>[2x]EPCVEVVPNITYQCMELNFYKIPDNLPFSTKNLDLSFNPLRHLGSYSFFSFPELQVLDLSRCEIQTIEDGAYQSLSHLSTLILTGNPIQSLALGAFSGLSSLQKLVAVETNLASLENFPIGHLKTLKELNVAHNLIQSFKLPEYFSNLTNLEHLDLSSNKIQSIYCTDLRVLHQMPLLNLSLDLSLNPMNFIQPGAFKEIRLHKLTL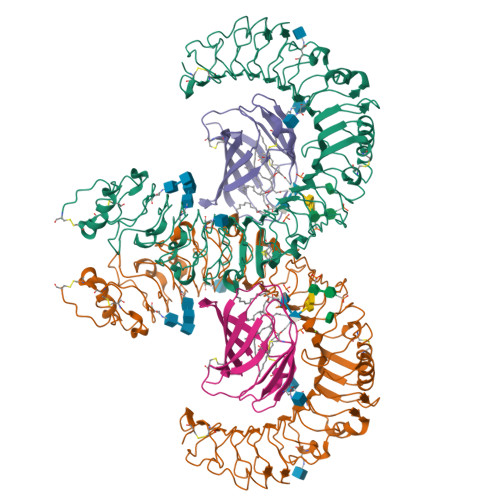RNNFDSLNVMKTCIQGLAGLEVHRLVLGEFRNEGNLEKFDKSALEGLCNLTIEEFRLAYLDYYLDDIIDLFNCLTNVSSFSLVSVTIERVKDFSYNFGWQHLELVNCKFGQFPTLKLKSLKRLTFTSNKGGNAFSEVDLPSLEFLDLSRNGLSFKGCCSQSDFGTTSLKYLDLSFNGVITMSSNFLGLEQLEHLDFQHSNLKQMSEFSVFLSLRNLIYLDISHTHTRVAFNGIFNGLSSLEVLKMAGNSFQENFLPDIFTELRNLTFLDLSQCQLEQLSPTAFNSLSSLQVLNMSHNNFFSLDTFPYKCLNSLQVLDYSLNHIMTSKKQELQHFPSSLAFLNLTQNDFACTCEHQSFLQWIKDQRQLLVEVERMECATPSDKQGMPVLSLNITCQMNK;>[2x]QKQYWVCNSSDASISYTYCDKMQYPISINVNPCIELKGSKGLLHIFYIPRRDLKQLYFNLYITVNTMNLPKRKEVICRGSDDDYSFCRALKGETVNTTISFSFKGIKFSKGKYKCVVEAISGSPEEMLFCLEFVILHQPNSN2,6-bis(fluoranyl)-N-[3-[5-[2-[(3-methylsulfonylphenyl)amino]pyrimidin-4-yl]-2-morpholin-4-yl-1,3-thiazol-4-yl]phenyl]benzenesulfonamide | C30 H26 F2 N6 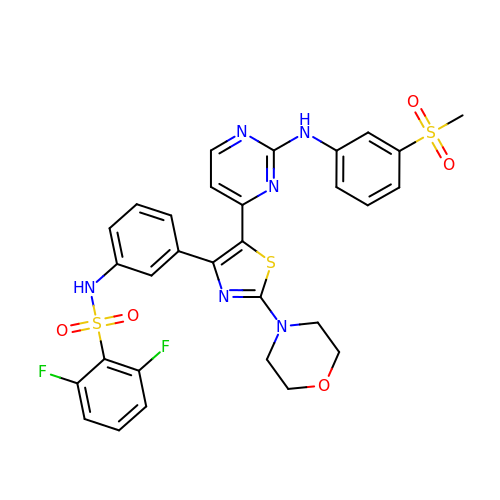O5 S3 | POWKQVBMRCSBOT-UHFFFAOYSA-N> 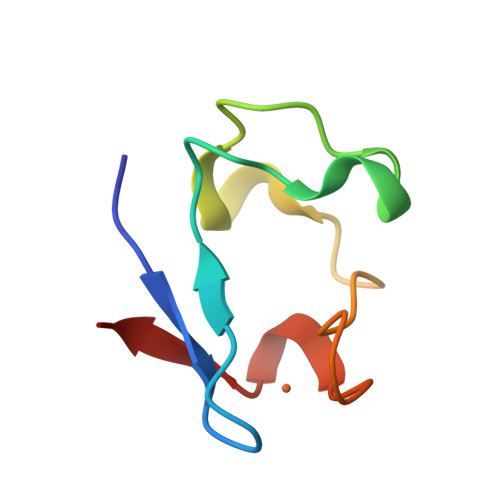MDIYVCTVCGYEYDPAKGDPDSGIKPGTKFEDLPDDWACPVCGASKDAFEKQ> GSTDSNNGYKELTMDGKHTVPYTISVDGITALHRTYFVFP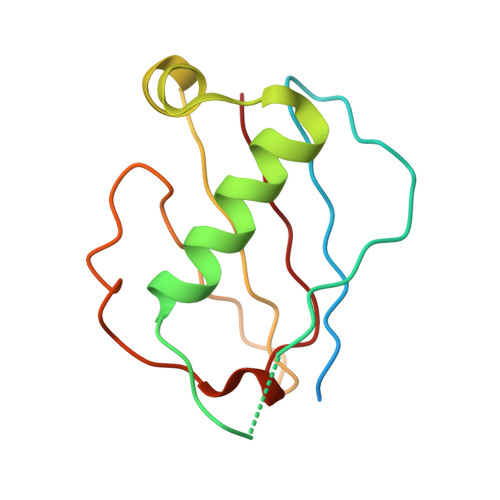ENKKVLYQEIDSKVKNELASQRGVTTEKINNAQTATYTLTLNDGNKKVVNLKKNDDAKNSIDPSTIKQIQIVVK3,3',3'',3'''-[3,8,13,17-tetrakis(carboxymethyl)porphyrin-2,7,12,18-tetrayl]tetrapropanoic 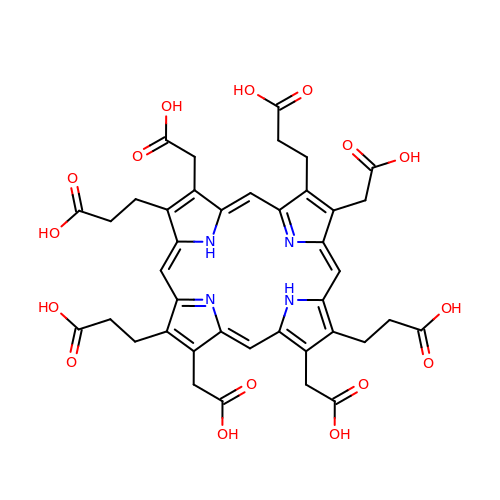acid | C40 H38 N4 O16 | VZVFNUAIRVUCEW-XFMUOGEMSA-N>MDVFAKHAVSLESPAVRHYEITPSDSTDLARRPRALRVQTGGTLVLRDETGITVTYTVFAGEILPVRPVRVLATGTTATAVGWE[11x];>[29x]MPEGADPVAEVKTALAGFLKEVKGFQDDVKTRLQQQEERVTMLQTKTYAGRHALAAAATEEAPHQKAFAAYLRTGDDDGLRGLSLEGKALNSAVAAEGGYLVDPQTSETIRGVLRSTASLRQIASVVNVEATSFDVLVDKTDMGSGWASETAALSETATPQIDRITIPLHELAAMPKASQRLLDDSAFDIETWLANRIADKFARAEAAAFISGDGVDKPTGFLTKTKVANGAWAWGSLGYVATGAAGDFAAVNASDAVVDLVYALGAEYRANASFVMNSKTAGAVRKMKDADGRFLWADSLAAGEPARLMGYPVLIAEDMPDIAANAYAIAFGDFGNGYTIAERPDLRVLRDPFSAKPHVLFYASKRVGGDVSDFAAIKLLKFAAS;>[2x]MIALGLGLGLAANGGPALRRYAVNGVAPVAVLDFERHFLSHPLALTRATSATYADALRAVQTAPADTPRYDYSTGKRALLLEASATNLLPNSAQFEAASWGKTRASVLANAALAPNGTMTADKLVEDTSNNSHFVARTGTQIAAGTSVTASIFVKAAERRWFALVTADSANAFRTTYFDLQTGTLGVVSQGAAGHVAQIVAAGNGWYRCSVTQTQAASGNFNFYPSVASANGATSYPGDGASGLYLWGAQLEAGAAVSSVIPTEAAAVTRAADLASVAVAAGSYDLRRVDAAGTAVTKGVAHPGGALTIGAGSLYLLSLFPAGAL

Gene transfer agents (GTAs) are DNA-containing phage-like particles produced by some species of bacteria and archaea. The genes encoding proteins that form Rhodobacter capsulatus GTA particles (RcGTA) are derived from phage DNA, which has been integrated into the bacterial genome. Here, we use cryo-electron microscopy (cryo-EM) to determine the structures of RcGTA before and after DNA ejection, and to visualize the interactions of RcGTA with R. capsulatus cells. Particles of RcGTA have heads with a diameter of 38-nm and 49-nm long tails.

The structure of the native RcGTA head with imposed fivefold symmetry has been determined to a resolution of 3.6 Å. Unlike the phage heads that are isometric or prolate, the capsid of RcGTA is oblate with the shortened dimension along the tail axis. The organization of the RcGTA capsid is derived from a T = 3 quasi-icosahedral lattice; however, it lacks five hexamers of major capsid proteins in its central part, which results in a shortening of the head. The volume for packaging DNA in the oblate head is 35% smaller than that of the corresponding T = 3 icosahedral head. The formation of the oblate head of RcGTA requires conformational adjustments of quasi-hexamers of major capsid proteins positioned on the twofold axes of the oblate head relative to the quasi-hexamers positioned on the threefold axes of the T = 3 quasi-icosahedral capsid. By contrast, the quasi-hexamers on twofold axes of the oblate capsid are bent to enable seamless closure of the oblate head. The quasi-hexamers on twofold axes of the oblate head contain subunits in three conformations: two subunits binding to pentamers from different directions, and one binding to a hexamer of capsid proteins. The surface of the RcGTA head is decorated with eleven 70-Å long head spikes attached to pentamers of major capsid proteins. Each head spike is composed of a pentamer of base proteins Rcc01079, and a single subunit of head fiber protein Rcc01080. Base proteins attach to the capsid by the N-termini, each of which binds to axial domains of two adjacent major capsid proteins within a pentamer.U2AF2 is a critical pre-mRNA splicing factor for the early stage of spliceosome assembly at the major class of 3′ splice sites. Two central RNA recognition motifs (RRM1 and RRM2) recognize a polypyrimidine consensus sequence (Py tract) composed primarily of uridines and at lower frequencies, cytidines. Structures of the U2AF2 RNA binding domain show an “open”, side-by-side conformation of the RRMs binds to uridine-rich Py tracts. Considering that the NDD-affected residues are located near the RNA interface of U2AF2 structures, here we investigated the hypothesis that disrupted U2AF2–RNA interactions could contribute to altered pre-mRNA splicing by the recurrent NDD-associated variants. De novo mutations affecting the pre-mRNA splicing factor U2AF2 are associated with developmental delays and intellectual disabilities, yet the molecular basis is unknown. To address this question, we determined the X-ray crystal structures of Arg149Trp- and Arg150His-substituted U2AF212L bound to Py tract oligonucleotides at 1.4 Å resolutions.

The Arg149Trp, Arg150His, and Arg150Cys substitutions decreased the apparent binding affinity of U2AF212L for this consensus site by approximately three-, four-, and five-fold. The sequence of the cocrystallized Py tract (5′-phosphoryl-UU(dU)U(5Br-dU)CC-3′) corresponds to a 3′ splice site of the AdML transcript, a well-characterized substrate for in vitro pre-mRNA splicing (e.g.,9,16). For the Arg149Trp U2AF212L variant, the bulky tryptophan disordered four N-terminal residues of U2AF212L as well as the Arg146 side chain, which lacked detectable electron density at 1σ contour level. Although the WT Arg149 did not contact the bound oligonucleotide, the nearby Arg146 side chain interacted with the terminal pyrimidine-O2 atom. In the Arg149Trp mutant structure, the Gln147 side chain flips to replace the former Arg146–nucleobase hydrogen bond. Neither of the amino acid substitutions significantly perturbed the other site–i.e., Arg149Trp has little effect on Arg150, and Arg150His had little effect on Arg149. Instead, the NDD-associated substitutions converged on disrupting Arg146 interactions with the terminal nucleotide of the cocrystallized Py tract. The effects of the variants on U2AF2 – RNA interactions are unlikely to be sequence-specific, since Arg146 interacts similarly with either uridine or cytidine. Unlike WT, the Arg149Trp, Arg150Cys, or Arg150His U2AF2 variants are unable to detectably promote splicing of a minigene transcript in HEK293T cells.

> GPLGSQMTRQAWRLYVGNIPFGITEEAMMDFFNAQMRLGGLTQAPGNPVLAVQINQDKNFAFLEFRSVDETTQAMAFDGIIFQGQSLKIRRPHDYQPLPGMSENPSVYVPGVVSTVVPDSAHKLFIGGLPNYLNDDQVKELLTSFGPLKAFNLVKDSATGLSKGYAFCEYVDINVTDQAIAGLNGMQLGDKKLLVQRASVGAKN>EVIASGRLEKCVVDGVTEELDCQEKVVVTLTVGNGQSLQTEALEFSLSCLNSPDGRCPCSCSAADPTCACRDLAAPLRVSLTKSPLWASYPLQYLSSFNWKPLEVILRPSNKVCKDGDWEDSPTCGWFSQGGVRVADSQGFCCECSSSQVWDDTFGSSKERTRANLDCDFWSDPLDILIGRKPVSAHCLTFDPQWYSGYELGAASLQFEIAITVEVPTAPSPTTATTSATPRTNNSSSANSTNSTNSPAPQFLSPPAPSTREVLHLGPSVPLASSASRLLSAKLLGDLAMYTQLPAISNQVLMVPQPPAAAAATGSPLDALATNRSAWMLLDKTMLSMDGLACDKVGTGFSAFRYQPSGCGRAPQACLSGQLKDLWEADLARIADGRVPLYMITRFTGGSDTTLQSFSGGPLSFALPVTSHSQSLVTLSVAADGVRLVTNRSPGKITGAAVCRFAGTSCGGFEAVAARGYIYVNITNTGRLDSDYTLTVSNCSSNVRPIEARTLAVRAGSAASLDPPMELYVEDQAAAAARTCTVSLYDSVGAVTDSLTLSFYTNATQLHHHHHH[3x]

The single-pass transmembrane protein HAP2/GCS1 is essential for gamete fusion in organisms across eukaryotic kingdoms, and was likely the ancient sexual fusogen used by primitive eukaryotes before the eukaryotic radiation. Recent work on HAP2 from the green alga Chlamydomonas, the flowering plant Arabidopsis, and the ciliate Tetrahymena shows that HAP2 is, in common with fusogens used by certain enveloped viruses to enter host cells, a class II fusion glycoprotein. Class II fusogens are characterized by their mainly β-sheet-containing-domains I, II, and III (referred to here as D1, D2, and D3). As with viral class II proteins, HAP2 functions uni-directionally.

Here, we report a 2.6 Å trimeric, fusion-state crystal structure of Chlamydomonas HAP2 in which the fusion loops are completely resolved. Chlamydomonas HAP2 glycoprotein (ectodomain residues 23 – 582) with a C-terminal His tag was secreted from Drosophila S2 cells, purified by Ni-affinity chromatography and gel filtration, and crystallized. Three monomers in the asymmetric unit form a trimer and pack against one another through D1 and D2 at the 3-fold axis. In further similarity to other class II fusion-state structures, a U-turn between D1 and D3 enables D3 to pack against the outer faces of D1 and D2. D2.2 at the ‘apical’, narrower end of trimers bears three fusion helices, α1, η1, and α2, in fusion loops 1 and 2 between β-strands c and d. Each helix, α1 in loop 1, and η1 and α2 in loop 2, displays a set of two to three hydrophobic residues that project apically. The Arg185 sidechain guanido group docks through six hydrogen bonds to its carbonyl cage formed by backbone and sidechain carbonyl oxygens in the core of subdomain D2.2. In the crystal structure, however, D2.2 splays away from the 3-fold axis so that the 3-helix fusion surfaces of monomers are separated from one another by solvent. Either as a consequence of omission of protease treatment here, differences in the crystal lattice, or higher resolution, we can visualize 50 more residues per monomer. Because of the large hydrophilic surface exposed on the faces of each monomer surrounding the 3-fold axis, deformation of lipids to fit into this large cavity, or the presence of water in the cavity, would limit the depth to which HAP2 trimers could insert in the hydrophobic core of the membrane bilayer during membrane fusion. These apparent barriers raise the possibility that our crystal structure represents an early fusion state of HAP2 that precedes a more mature state in which reorientation could allow the fusion loops in each monomer to approach and close up at the 3-fold axis to form a common fusion surface.> MDVVVRLPDVAVPGEAVQASARQAVIHLVDIAGITSSTPADYATKNLYLWNNETCDALSAPVADWNDVSTTPTGSDKYGPYWVIPLTKESGCINVIVRDGTNKLIDSDLRVSFSDFTDRTVSVIAGNSAVYDSRADAFRAAFGVALADAHWVDKTTLLWPGGENKPIVRLYYSHSSKVAADSNGEFSDKYVKLTPTTVSQQVSMRFPHLASYPAFKLPDDVNVDELLQGETVAIAAESDGILSSATQVQTAGVLDDTYAAAAEALSYGAQLTDSGVTFRVWAPTAQQVELVIYSADKKVIASHPMTRDSASGAWSWQGGSDLKGAFYRYAMTVYHPQSRKVEQYEVTDPYAHSLSTNSEYSQVVDLNDSALKPEGWDGLTMPHAQKTKADLAKMTIHESHIRDLSAWDQTVPAELRGKYLALTAQESNMVQHLKQLSASGVTHIELLPVFDLATVNEFSDKVADIQQPFSRLCEVNSAVKSSEFAGYCDSGSTVEEVLTQLKQNDSKDNPQVQALNTLVAQTDSYNWGYDPFHYTVPEGSYATDPEGTARIKEFRTMIQAIKQDLGMNVIMDVVYNHTNAAGPTDRTSVLDKIVPWYYQRLNETTGSVESATCCSDSAPEHRMFAKLIADSLAVWTTDYKIDGFRFDLMGYHPKAQILSAWERIKALNPDIYFFGEGWDSNQSDRFEIASQINLKGTGIGTFSDRLRDAVRGGGPFDSGDALRQNQGVGSGAGVLPNELTTLSDDQARHLADLTRLGMAGNLADFVLIDKDGAVKRGSEIDYNGAPGGYAADPTEVVNYVSKHDNQTLWDMISYKAAQEADLDTRVRMQAVSLATVMLGQGIAFDQQGSELLRSKSFTRDSYDSGDWFNRVDYSLQDNNYNVGMPRSSDDGSNYDIIARVKDAVATPGETELKQMTAFYQELTALRKSSPLFTLGDGATVMKRVDFRNTGADQQTGLLVMTIDDGMQAGASLDSRVDGIVVAINAAPESRTLQDFAGTSLQLSAIQQAAGDRSLASGVQVAADGSVTLPAWSVAV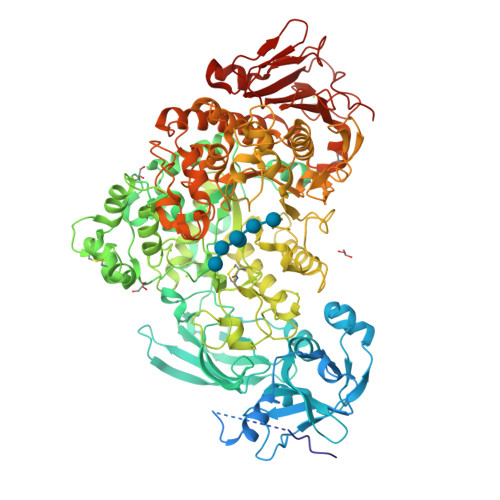LELPQGESQGAGLPVSSK>AAPTAYTPLDVAQAYQFPEGLDGQGQCIAIIELGGGYDEASLAQYFASLGVPAPQVVSVSVDGASNQPTGDPSGPDGHVELDIEVAGALAPGAKFAVYFAPNTDAGFLDAITTAIHDPTLKPSVVSISWGGPEDSWTSAAIAAMNRAFLDAAALGVTVLAAAGNSGSTDGEQDGLYHVDFPAASPYVLACGGTRLVASGGRIAQETVWNDGPDGGATGGGVSRIFPLPAWQEHANVPPSANPGASSGRGVPDLAGNADPATGYEVVIDGEATVI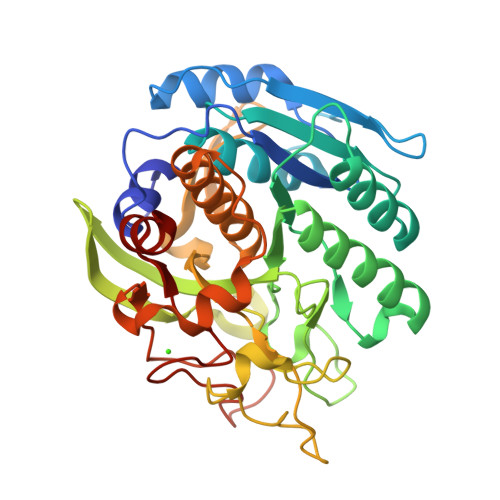GGTSAVAPLFAALVARINQKLGKAVGYLNPTLYQLPADVFHDITEGNNDIANRAQIYQAGPGWDPCTGLGSPIGVRLLQALLPS[2x]>MSAIPFSTDDCSQDETLPSLLLIDEAAAVLGRMIQGLRTGIPYIHTENDSIKANPILRTALWQAAYVLEKAYRRRYRVPWTARRYMRELTPRQDGRNANREAVMAKEFPPGAELNSDHPVQEILPAMIIDAEDHILFCYLPSCVSPAIMTIIDAAVGTLATTKDGHLQKKSRAREGERARVEMQKVKGKGKQEEEGQEKLGANWREALDLFRQGACKMTPGVLTFAPAWWPVGHENQLPGPASTLKPPK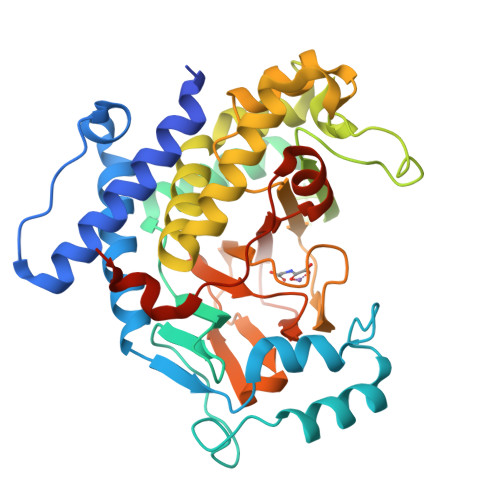GEGRMFLSDIPIASALVGAILAQINQPLFESGVKVLRELYSNSKLTKDHSTVSKIIEIWFSPFSSLSLIVNRATPIHRDTSGPIEGMDILVTGGNYSNGVLVTPSFNRRWTYNPGCVVALLGKLVLHGVPEVDGERYCMAHFWRERLFDAAGVPFPYPSKWQESYTNIPEALQWHRDNVTR[4x]> MSV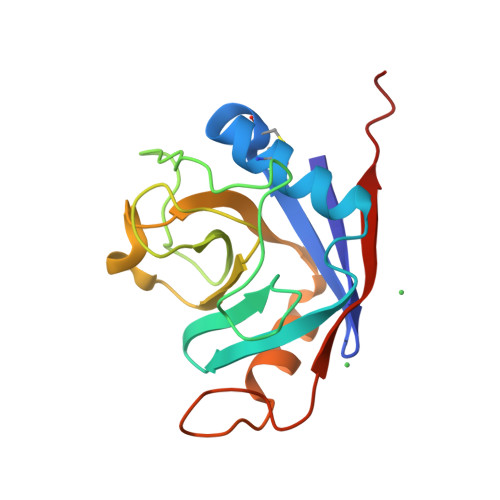TLHTDVGDIKIEVFCERTPKTCENFLALCASNYYNGCIFHRNIKGFMVQTGDPTGTGRGGNSIWGKKFEDEYSEYLKHNVRGVVSMANNGPNTNGSQFFITYGKQPHLDMKYTVFGKVIDGLETLDELEKLPVNEKTYRPLNDVHIKDITIHANPFAQ> CACACG;> CGTGT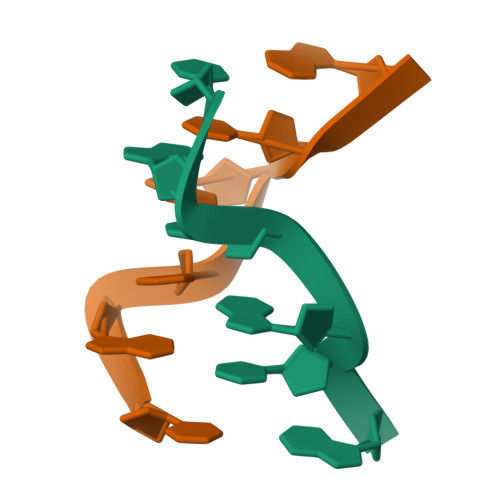G> VDMFLYNLTLQRATGISFAIHGNFSGTKQQEIVVSRGKILELLRPDPNTGKVHTLLTVEVFGVIRSLMAFRLTGGTKDYIVVGSDSGRIVILEYQPSKNMFEKIHQETFGKSGCRRIVPGQFLAVDPKGRAVMISAIEKQKLVYILNRDAAARLTISSPLEAHKANTLVYHVVGVDVGFENPMFACLEMDYEEADNDPTGEAAANTQQTLTFYELDLGLNHVVRKYSEPLEEHGNFLITVPGGSDGPSGVLICSENYITYKNFGDQPDIRCPIPRRRNDLDDPERGMIFVCSATHKTKSMFFFLAQTEQGDIFKITLETDEDMVTEIRLKYFDTVPVAAAMCVLKTGFLFVASEFGNHYLYQIAHLGDDDEEPEFSSAMPLEEGDTFFFQPRPLKNLVLVDELDSLSPILFCQIADLANEDTPQLYVACGRGPRSSLRVLRH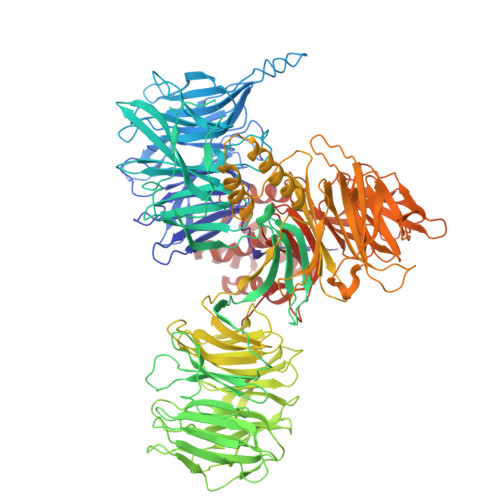GLEVSEMAVSELPGNPNAVWTVRRHIEDEFDAYIIVSFVNATLVLSIGETVEEVTDSGFLGTTPTLSCSLLGDDALVQVYPDGIRHIRADKRVNEWKTPGKKTIVKCAVNQRQVVIALTGGELVYFEMDPSGQLNEYTERKEMSADVVCMSLANVPPGEQRSRFLAVGLVDNTVRIISLDPSDCLQPLSMQALPAQPESLCIVEMGGTEKQDELGERGSIGFLYLNIGLQNGVLLRTVLDPVTGDLSDTRTRYLGSRPVKLFRVRMQGQEAVLAMSSRSWLSYSYQSRFHLTPLSYETLEFASGFASEQCPEGIVAISTNTLRILALEKLGAVFNQVAFPLQYTPRKFVIHPESNNLIIIETDHNAYTEATKAQRKQQMAEEMVEAAGEDERELAAEMAAAFLNENLPESIFGAPKAGNGQWASVIRVMNPIQGNTLDLVQLEQNEAAFSVAVCRFSNTGEDWYVLVGVAKDLILNPRSVAGGFVYTYKLVNNGEKLEFLHKTPVEEVPAAIAPFQGRVLIGVGKLLRVYDLGKKKLLRKCENKHIANYISGIQTIGHRVIVSDVQESFIWVRYKRNENQLIIFADDTYPRWVTTASLLDYDTVAGADKFGNICVVRLPPNTNDEVDSQKAEVIMNYHVGETVLSLQKTTLIPGGSESLVYTTLSGGIGILVPFTSHEDHDFFQHVEMHLRSEHPPLCGRDHLSFRSYYFPVKNVIDGDLCEQFNSMEPNKQKNVSEELDRTPPEVSKKLEDIRTRYAFDYKDDDDK Acetyl-CoA carboxylases (ACCs) have crucial roles in fatty acid biosynthesis and oxidation and are promising targets for drug discovery against diabetes, cancer and other diseases. ACC carries two distinct catalytic activities, biotin carboxylase (BC) and carboxyltransferase (CT), and its biotin is linked covalently to the biotin carboxyl carrier protein (BCCP). Although bacterial ACCs contain multiple subunits that support these different functions, most eukaryotic ACCs are single-chain, multi-domain enzymes with a molecular weight of ~250 kDa and are active as dimers and higher oligomers. The unique central region of ACC, with five domains (AC1–AC5, AC: ACC Central), is located at the sides, far away from the two active sites.

To illuminate the molecular basis for how phosphorylated Ser1157 (pSer1157) is recognized by ScACC, we determined the crystal structure at 2.9 Å resolution of domains AC3–AC5 with Ser1157 fully phosphorylated with our in vitro phosphorylation system. The loop containing pSer1157 is located in a groove at the interface between domains AC4 and AC5, with pSer1157 positioned in an electropositive pocket in domain AC4. The phosphate group interacts with the side chains of Arg1173, Arg1260, Tyr1113 and Ser1159, and these residues are well conserved among those eukaryotic ACCs that contain this phosphorylation site. To assess the functional importance of this binding site, we created the R1173A/R1260A double mutant and found that its catalytic activity was only mildly inhibited upon treatment with activated SNF1. The overall structure of the phosphorylated AC3–AC5 is nearly the same as that of unphosphorylated AC3–AC5 alone, with r.m.s. distance of 0.48 Å for their 402 equivalent Cα atoms. However, there is a large difference in the position of AC5 relative to AC3–AC4 compared with the structure of these domains in the holoenzyme. With domains AC3–AC4 in overlay between the structures of the (phosphorylated) AC3–AC5 and the holoenzyme, the orientation of AC5 differs by a rotation of 40°. Moreover, unphosphorylated Ser1157 in the holoenzyme structure is located in a different pocket, at the AC4–AC5 interface and ~16 Å away from pSer1157, suggesting a large conformational change for the loop containing Ser1157 upon its phosphorylation. The overall structure of phosphorylated AC3–AC5 is similar to that of phosphorylated AC1–AC5 of ScACC reported recently, with r.m.s. distance of 0.63 Å for 391 equivalent Cα atoms between them. The structure of AC3–AC5 alone represents the inactive conformation, which is stabilized by the phosphorylation of Ser1157.

>SVKERTEQIEHILKSSVVKVAYGSSNPKRSEPDLNILKDLIDSNYVVFDVLLQFLTHQDPVVTAAAAQVYIRRAYRAYTIGDIRVHEGVTVPIVEWKFQLPSAAFSTFPTVKSKMGMNRAVSVSDLSYVANSQSSPLREGILMAVDHLDDVDEILSQSLEVIPRHQSSSNGPAPDRSGSSASLSNVANVCVASTEGFESEEEILVRLREILDLNKQELINASIRRITFMFGFKDGSYPKYYTFNGPNYNENETIRHIEPALAFQLELGRLSNFNIKPIFTDNRNIHVYEAVSKTSPLDKRFFTRGIIRTGHIRDDISIQEYLTSEANRLMSDILDNLEVTDTSNSDLNHIFINFIAVFDISPEDVEAAFGGFLERFGKRLLRLRVSSAEIRIIIKDPQTGAPVPLRALINNVSGYVIKTEMYTEVKNAKGEWVFKSLGKPGSMHLRPIATPYPVKEWLQPKRYKAHLMHHHHHH[2x]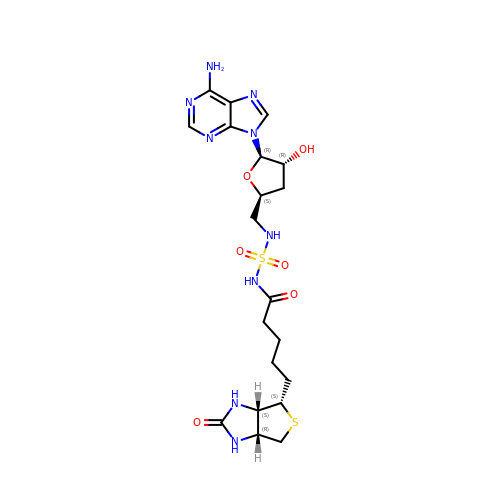3',5'-dideoxy-5'-[({5-[(3aS,4S,6aR)-2-oxohexahydro-1H-thieno[3,4-d]imidazol-4-yl]pentanoyl}sulfamoyl)amino]adenosine | C20 H29 N9 O6 S2 | CZQLNGUCLOAYQM-TVYLXWJSSA-N> GPMSRNDKEPFFVKFLKS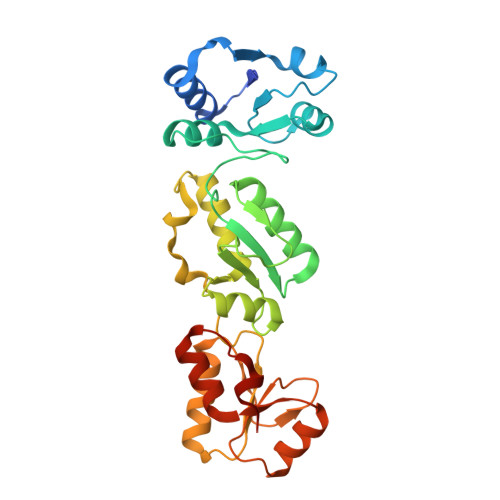SDNSKCFFKALESIKEFQSEEYLQIITEEEALKIKENDRSLYICDPFSGVVFDHLKKLGCRIVGPQVVIFCMHHQRCVPRAEHPVYNMVMSDVTISCTSLEKEKREEVHKYVQMMGGRVYRDLNVSVTHLIAGEVGSKKYLVAANLKKPILLPSWIKTLWEKSQEKKITRYTDINMEDFKCPIFLGCIICVTGLCGLDRKEVQQLTVKHGGQYMGQLKMNECTHLIVQEPKGQKYECAKRWNVHCVTTQWFFDSIEKGFCQDESIYKTEPRPEA>[2x]DTTPRRDAEYPPPELLEALKPLHDICLGKTGVTEEAIKKFSDEEIHEDEKLK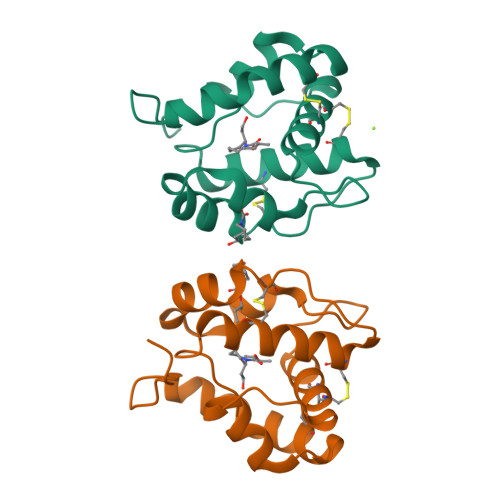CYMNCLFHEAKVVDDNGDVHLEKLHDSLPSSMHDIAMHMGKRCLYPEGETLCDKAFWLHKCWKQSDPKHYFLV> TKQTVETLMAGERIAEALELGMTDLNTIREWEEARQINPNIA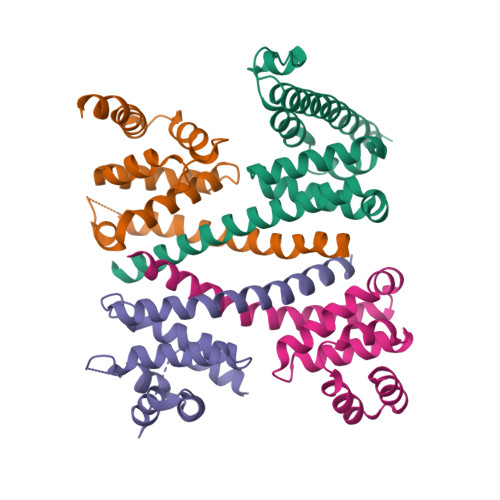PPQRNPIFVALGNIPAETYVLNTLQKIKPASLHDALLVLPFSTIPSLLTFLNLFAQRELNVPLTCRILFFVLKTHHKQIVASRTMRATLEKVRANLRAALRRQKDEMGFNIAALKVVSMQL;> LVEQEQTLENYIHAGAYRDAIVLALQLNHPGRLLNLFTNVVTTRNPDPDSLTGLKAVDDVLAKLSDEQIFQLLLRLRDWNTNARTAPVAQRVLWALFKSHPANKLSSLSVKGARGHKSLNEVLDAIKVYTERHYKRIEELVDESYLVEYTLR;> EGGQGLIEAALEAEEEQAEDDGVMAPIIDQLSADMMTLSLVPRSRWQTLLHIDIIKARNKPKEPPKAPEKAPFFLPPVGQNGISSLIPQEDAKAKKEKAAANGASRITKLDLTRQEQTFTSKLLVGGAKGDYTDFIEHLKALPPAAADLELRSLSIGNGDEATNELLHFIRALTSRLVARRDYELTQAWMTVFLRLHFDLIMENEELLQALGEWREHQARERDRLSELVGYCGGVVSFLRSPRT;> DNTVQFDPFDLNMEITPASTLAVLEKEKDYLKALVMAFRLNEAGLITRVYQAIPYTDIGLVVEQFPTVYVPRLLRFVAAQTEQSPHMEFCLLWIRALIDKHGPWLAANRGKVDVELRVVARAVAKMRDEIRRLADENVYMVDYLLNQAK>[2x]GTSHTVPTAQASLS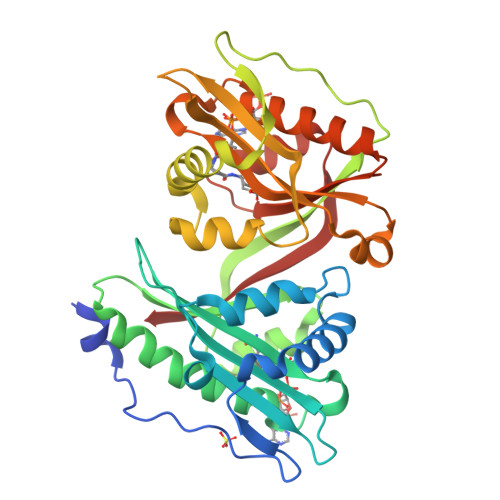ERVDAPDVVEIPSAGADLTWRAATKEDIPALFELWRAAGAVDHPTSLVMLDELEEEFDDDDFDPALDSVIAVDSLGRVVAFGSATVKSAHETVVWVALDGTVHPERRGEGIGSSVLRWQEQRGLQHLAESDECLPGWLASSAEEHAVWTIELFHRNGYESVRWWHELERDLAQPIPDVTLPEGIRIETYGPEWSEPTRDAHNEAFRDHWGSQPEAREDWEAAHRLSAFRADLSFVAVARDAAGQDIVVAYLLSDVNEEEWEANGYSFGFVDLLGVRRDWRGRKLAQALLTHAMRAYRHEGLQRAVLDVDADSPTGAVALYEGLGFSLVNRSISLIKQF>MSIRSLGYLRIEATDMAAWREYGLKVLGMVEGKGAPEGALYLRMDDFPARLVVVPGEHDRLLEAGWECANAEGLQEIRNRLDLEGTPYKEATAAELADRRVDEMIRFADPSGNCLEVFHGTALEHRRVVSPYGHRFVTGEQGMGHVVLSTRDDAEALHFYRDVLGFRLRDSMRLPPQMVGRPADGPPAWLRFFGCNPRHHSLAFLPMPTSSGIVHLMVEVEQADDVGLCLDRALRRKVP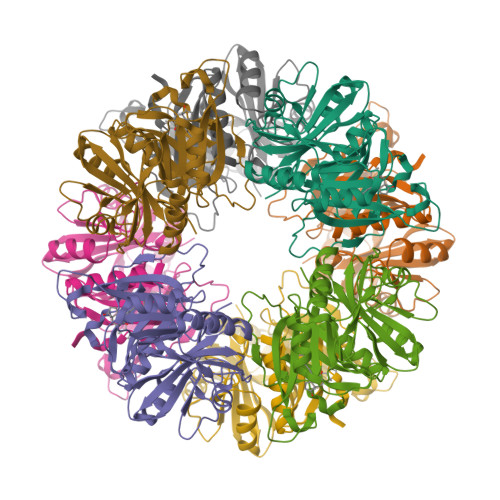MSATLGRHVNDLMLSFYMKTPGGFDIEFGCEGRQVDDRDWIARESTAVSLWGHDFTVGARG[2x]>[2x]DNSYKMDYPEMGLCIIINNKNFHKSTGMTSRSGTDVDAANLRETFRNLKYEVRNKNDLTREEIVELMRDVSKEDHSKRSSFVCVLLSHGEEGIIFGTNGPVDLKKITNFFRGDRCRSLTGKPKLFIIQACRGTELDCGIET;>[2x]CHKIPVE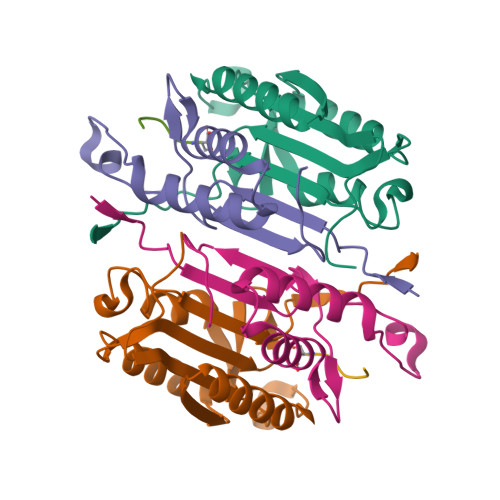ADFLYAYSTAPGYYSWRNSKDGSWFIQSLCAMLKQYADKLEFMHILTRVNRKVATEFESFSFDATFHAKKQIPCIVSMLTKELYFYHH;>XVDPVD[2x]> PKPWLGAQPATVVTPGVNVTLRCRAPQPAWRFGLFKPGEIAP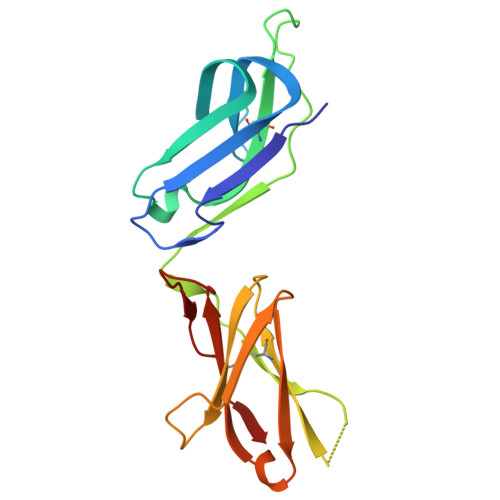LLFRDVSSELAEFFLEEVTPAQGGIYRCCYRRPDWGPGVWSQPSDVLELLVTEELPRPSLVALPGPVVGPGANVSLRCAGRLRNMSFVLYREGVAAPLQYRHSAQPWADFTLLGARAPGTYSCYYHTPSAPYVLSQRSEVLVI2-(3-bromophenyl)-6-chloroquinoline-4-carboxylic acid 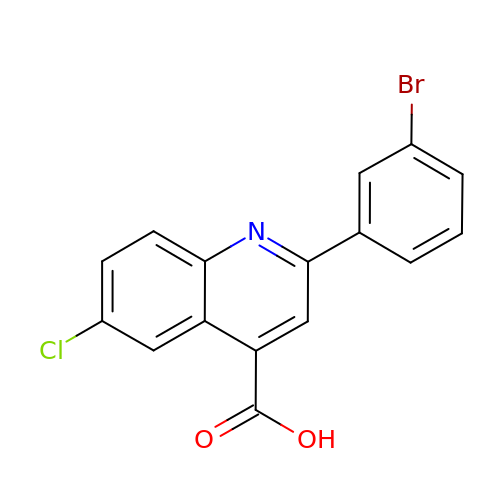| C16 H9 Br Cl N O2 | UEYRXZBCYPCXSJ-UHFFFAOYSA-N>[2x]GSHMGRFADFFRIETEIQRLDNPAGILANGKKCDFTGACDPVVTAFLDLESPLSPWPGSVAASKWKTIFEATDQNSPTIGRSVIRDMCGGSAS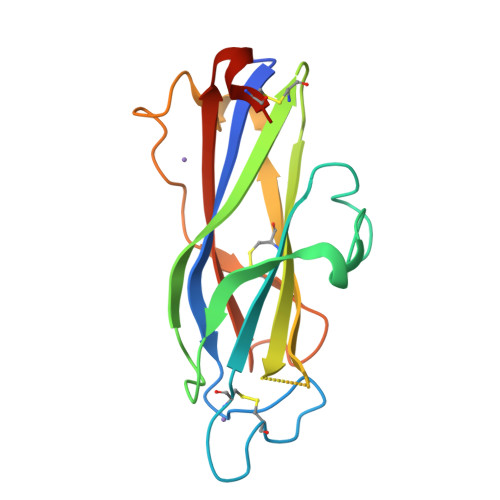NVNLRVLVNDADSLSSQDEIGKFSCLFQLDARDVAMDSLSAQWGPSTECTAEAQQGKIRLFARRRAFEIPSTSCRAPSSL>GMSSLPAVYIVSSARTPVGSFLGSLSSLTAPQLGAHAIKAALAKVDGLKPSDVQEVFFGNVISANVGQNPARQCALGAG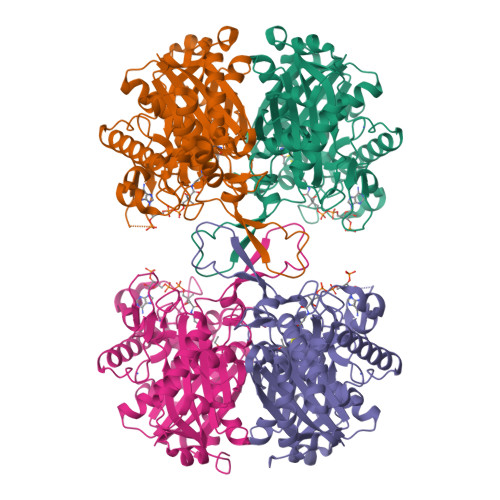LEESTICTTVNKVCASGLKAIILGAQTIMTGNADVVVAGGTESMSNAPHYLPNLRTGAKYGHQSLVDGIMKDGLTDAGKQELMGLQAEECAQDHGFSREQQDEYAIRTYEKAQAAQKAGLFDEEIAPIQLPGFRGKPDVTVTQDEEPKNLNPEKLRAIKPAFIPGSGTVTAPNSSPLNDGAAAVVLVSEAKLKELNLKPVAKILGWGDAAQQPSKFTTAPALAIPKALKHAGVGQDAIDAFEINEAFSVVALANMKLLGIPEEKVNLHGGAVAIGHPIGASGARILTTLLGVLKAKKGKLGCAGICNGGGGASALVVELL[4x]>HHHHHHSSGLVPRGSHMASMINIISRLQEVFGHAIKAAYPDLENPPLLVTPSQQAKFGDYQCNSAMGISQMLKTKEQKVNPREIAENITKHLPDNECIEKVEIAGPGFINVHLRKDFVSEQLTSLLVNGVQLPALGENKKVIVDFSSPNIAKEMHVGHLRSTIIGESISRLFEFAGYDVLRLNHVGDWGTQFGMLIAHLQDKFPDYLTVSPPIGDLQVFYKESKKRFDTEEEFKKRAYQCVVLLQGKNPDITKAWKLICDVSRQELNKIYDALDVSLIERGESFYQDRMNDIVKEFEDRGFVQVDDGRKIVFVPGCSIPLTIVKSDGGYTYDTSDLAAIKQRLFEEKADMIIYVVDNGQSVHFQTIFAA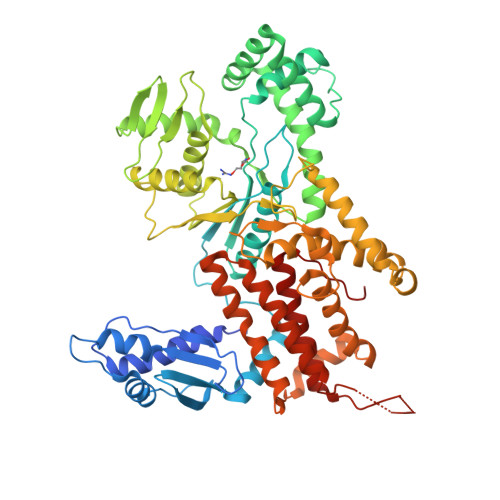AQMIGWYDPKVTRVFHAGFGVVLGEDKKKFKTRSGETVRLMDLLGEGLKRSMDKLKEKERDKVLTAEELNAAQTSVAYGCIKYADLSRNRLNDYIFSFDKMLDDRGNTAAYLLYAFTRIRSIARLANIDEEMLQKAARETKILLDHEKEWKLGRCILRFPEILQKILDDLFLHTLCDYIYELATAFTEFYDSCYCVEKDRQTGKILKVNMWRMLLCEAVAAVMAKGFDILGIKPVQRM[2x]4-[(3,5-DICHLORO-4-METHOXYPHENYL)AMINO]-6-METHOXY-7-[3-(4-METHYLPIPERAZIN-1-YL)PROPOXY]QUINOLINE-3-CARBONITRILE 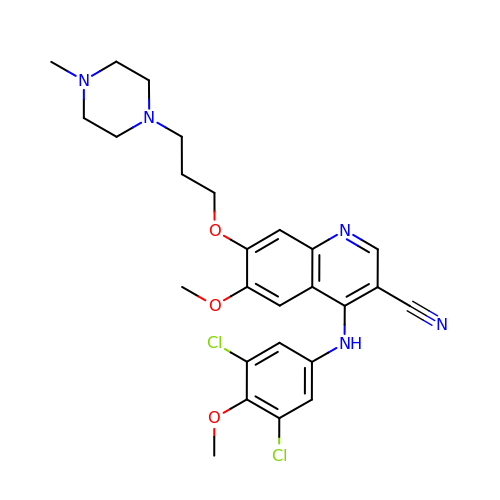| C26 H29 Cl2 N5 O3 | YCLIWTLPTXAGPQ-UHFFFAOYSA-N> GAMDPSEALQRPVASDFEPQGLSEAARWNSKENLLAGPSENDPNLFVALYDFVAS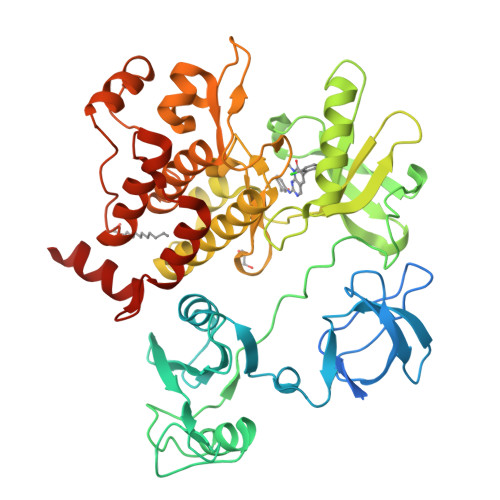GDNTLSITKGEKLRVLGYNHNGEWCEAQTKNGQGWVPSNYITPVNSLEKHSWYHGPVSRNAAEYLLSSGINGSFLVRESESSPGQRSISLRYEGRVYHYRINTASDGKLYVSSESRFNTLAELVHHHSTVADGLITTLHYPAPKRNKPTIYGVSPNYDKWEMERTDITMKHKLGGGQYGEVYEGVWKKYSLTVAVKTLKEDTMEVEEFLKEAAVMKEIKHPNLVQLLGVCTREPPFYIITEFMTYGNLLDYLRECNRQEVSAVVLLYMATQISSAMEYLEKKNFIHRNLAARNCLVGENHLVKVADFGLSRLMTGDTYTAHAGAKFPIKWTAPESLAYNKFSIKSDVWAFGVLLWEIATYGMSPYPGIDLSQVYELLEKDYRMERPEGCPEKVYELMRACWQWNPSDRPSFAEIHQAFETMFQESSISDEVEKELGKRGT>MHHHHHHMMQEPLTKERLISDWNSNVSVAVARTTAIAKSSDASLVQFLAADAAATTKSTANVLKQIEPLITQPAEREILDKIMQVRKTYIASRDKVSQLKADGMAEEAESTLINSYVPAAQGYLKLLGELLNLQRASLDAKAAEVEQIESSS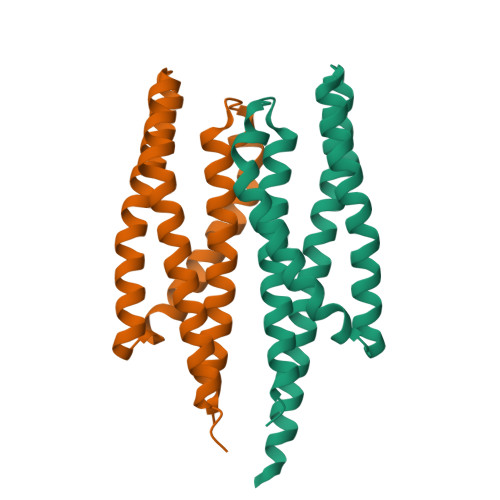RT[8x]DNA gyrase is the only type II topoisomerase capable of catalyzing DNA supercoiling, in a reaction driven by ATP hydrolysis. DNA gyrase consists of two subunits, GyrA and GyrB (97 kDa and 90 kDa, respectively, in Escherichia coli), forming an A2B2 complex in the active enzyme. The N-terminal domain of GyrB is the site of ATP hydrolysis, while DNA cleavage and strand passage occur at the interface between the C-terminal domain of GyrB and the N-terminal domain of GyrA. A new GyrA NTD fragment was constructed with a view of obtaining a crystal structure of SD8 bound to GyrA in an alternative conformation that would be representative of the situation at lower ligand concentrations. This smaller 55-kDa NTD fragment of GyrA (GyrA55), comprising residues 30–522 of the 875-amino-acid wild-type sequence (compared with residues 2–522 for GyrA59), crucially lacks residues spanning Leu17 to Asp23 that have been identified as providing 10 of the 12 protein–protein hydrogen bonds responsible for stabilizing the tetramer at the dimer–dimer interface in the crystal structure of the GyrA59–SD8 complex.

Comparisons within this structure reveal some conformational flexibility, with overall RMSD values up to 1.28 Å for monomer–monomer superpositions and up to 1.37 Å for dimer–dimer superpositions. Superposition of each homodimer with a homodimer generated from the apoGyrA59 crystal structure (which has a single monomer in the ASU) gives RMSD values of 0.87 and 1.20 Å, indicating that there is less variation across these two structures than within the apoGyrA55 structure. Additionally, there are a number of side-chain rearrangements around the SD8-binding site, but most of these are relatively minor, the exception being Arg91, which is disordered in the apoGyrA55 structure, with either no clear density for the guanidinium group and/or high temperature factors in each of the four monomers, suggesting that it is highly mobile in the absence of SD8. The structures presented in this work fit with the group of type II topoisomerase structures that have a closed exit gate and no DNA bound; that is, they are consistent with the existing structures. In addition, we have also presented the high-resolution structure of apoGyrA55 that has allowed us to describe specific conformational changes brought on by the action of SD8 binding to gyrase.

>[4x]VGRALPDVRDGLKPVHRRVLYAMNVLGNDWNKAYKKSARVVGDVIGKYHPHGDSAVYDTIVRMAQPFSLRYMLVDGQGNFGSIDGDSAAAMRYTEIRLAKIAHELMADLEKETVDFVDNYDGTEKIPDVMPTKIPNLLVNGSSGIAVGMATNIPPHNLTEVINGCLAYIDDEDISIEGLMEHIPGPDFPTAAIINGRRGIEEAYRTGRGKVYIRARAEVEVDAKTGRETIIVHEIPYQVNKARLIEKIAELVKEKRVEGISALRDESDKDGMRIVIEVKRDAVGEVVLNNLYSQTQLQVSFGINMVALHHGQPKIMNLKDIIAAFVRHRREVVTRRTIFELRKARDRAHILEALAVALANIDPIIELIRHAPTPAEAKTALVANPWQLGNVAAMLERAGDDAARPEWLEPEFGVRDGLYYLTEQQAQAILDLRLQKLTGLEHEKLLDEYKELLDQIAELLRILGSADRLMEVIREELELVREQFGDKRRTEIT> MLEQPYLDLAKKVLDEGHFKPDRTHTGTYSIFGHQMRFDLSKGFPLLTTKKVPFGLIKSELLWFLHGDTNIRFLLQHRNHIWDEWAFEKWVKSDEYHGPDMTDFGHRSQKDPEFAAVYHEEMAKFDD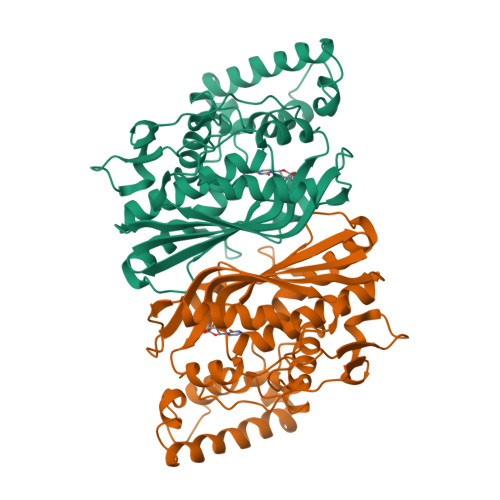RVLHDDAFAAKYGDLGLVYGSQWRAWHTSKGDTIDQLGDVIEQIKTHPYSRRLIVSAWNPEDVPTMALPPCHTLYQFYVNDGKLSLQLYQRSADIFLGVPFNIASYALLTHLVAHECGLEVGEFIHTFGDAHLMVNHLDQIKEQLSRTPRPAPTLQLNPDKHDIFDFDMKDIKLLNYDPYPAIKAPVAV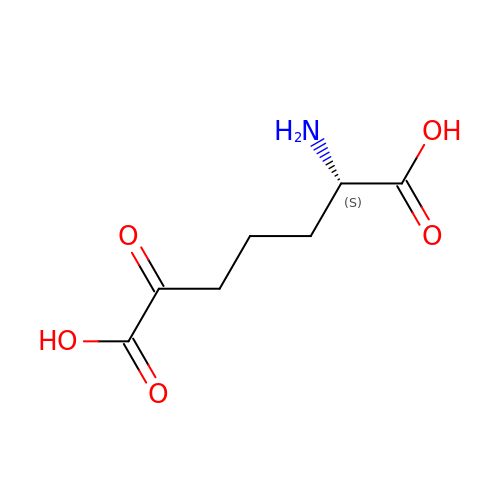2-AMINO-6-OXOPIMELIC ACID | C7 H11 N O5 | UKCSFKLWNHUBDY-BYPYZUCNSA-N Here, we report that bacterial, archaeal, and eukaryotic conserved histidine α-helical (CHAD) domains are specific polyP-binding modules. All CHAD domains fold into two 4-helix bundles with up-down-up-down topology. Analysis of the surface charge distribution in the different CHAD domains revealed a highly basic central cavity, which is surrounded by two basic surface patches on each side. The basic amino acids contributing to these surface patches are highly conserved among different CHAD proteins.

We identified an expressed CHAD domain–containing protein in the plant R. communis L. (RcCHAD), which represents the only CHAD domain currently known in plants. We selected CHAD domain–containing proteins belonging to the three kingdoms of life: archaea (Sulfolobus solfataricus; termed SsCHAD hereafter), bacteria (Chlorobium tepidum; CtCHAD), and eukaryota (Ricinus communis or castor bean; RcCHAD). We, thus, used the moderate anomalous signal present in the native RcCHAD dataset to locate a single Zn2+ ion. The structure was solved using the single-wavelength anomalous dispersion method, and the refined model revealed a Zn2+ ion tetrahedrally coordinated by His50 and His136 originating from two symmetry-related RcCHAD molecules. Although we found a Zn2+ ion coordinated by two histidine residues in our RcCHAD structure, the contributing histidines are not conserved among CHAD family proteins, and no metal ions could be located in our CtCHAD and ygiF structures. This makes it unlikely that CHAD domains are metal-binding proteins. Notably, helices α4/α5 and α10/α11 are protruding the bundle cores in the RcCHAD and CtCHAD structures, forming a small pore in the center of the domain, which we find to be absent in our ygiF structure. This rationalizes the presence of “long” (∼300 amino acids, e.g., RcCHAD and CtCHAD) and “short” (∼200 amino acids, e.g., ygiF and SsCHAD) CHAD domains. RcCHAD and SsCHAD bind polyP with a one-to-one kinetics and with a KD of 6 μM and 45 nM, respectively. We found that the fusion protein specifically localized to the nucleus and nucleolus of hypocotyl and root cells.

> GAMLVRETGHAPFRAQALALDADAALSEAFPAILGNCLEHIQRNEVAVIEGHDPETLHQMRVGVRRLRSALKLFDAVAPCPPALQDDISWLGTELGAARDWDVLLASTLPRIDGAPAGANGLLELNALVQKIAQAKRHAAAQALLSPRYTRLMLTLGAWMLETAPLLDGSAAHFSRQIMQHLHKSLLKRAARMQDDDAASAHRTRIATKRGRYALEFFHGLYRSKSTRAYLKALAATQEELGRHNDLVVAGRLLQELAQQQPQAAEAVQFARGYLLAQQAMRPADLDAIRAGLHALRAPQLRH>[2x]MSRKPLIAGNWKMNLNHYEAIALVQKIAFSLPDKYYDRVDVAVIPP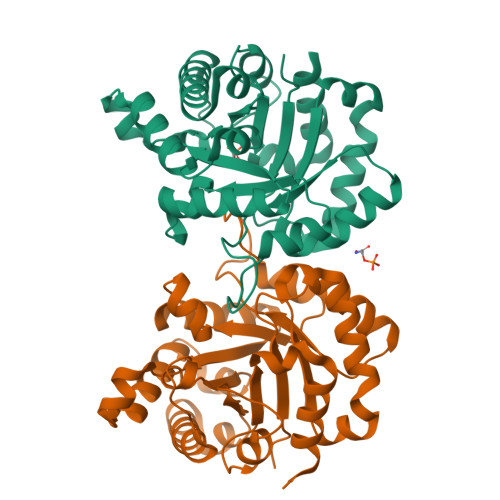FTDLRSVQTLVDGDKLRLTYGAQDLSPHDSGAYTGDVSGAFLAKLGCSYVVVGHSERRTYHNEDDALVAAKAATALKHGLTPIVCIGEHLDVREAGNHVAHNIEQLRGSLAGLLAEQIGSVVIAYEPVWAIGTGRVASAADAQEVCAAIRKELASLASPRIADTVRVLYGGSVNAKNVGDIVAQDDVDGGLVGGASLDGEHFATLAAIAAGGPLPHHHHHH>[2x]LSECKTGNGKNYRGTMSKTKNGITCQKWSSTSPHRPRFSPATHPSEGLEENYCRNPDNDPQGPWCYTTDPEKRYDYCDILECEEECMHCSGENYDGKISKTMSGLECQAWDSQSPHAHGYIPSKFPNKNLKKNYCRNPDRELRPWCFTTDPNKRWELCDIPRCTTPPPSSGPTYQCLKGTGENYRGNVAVTVSGHTCQHWSAQTPHTHERTPENFPCKNLDENYCRNPDGK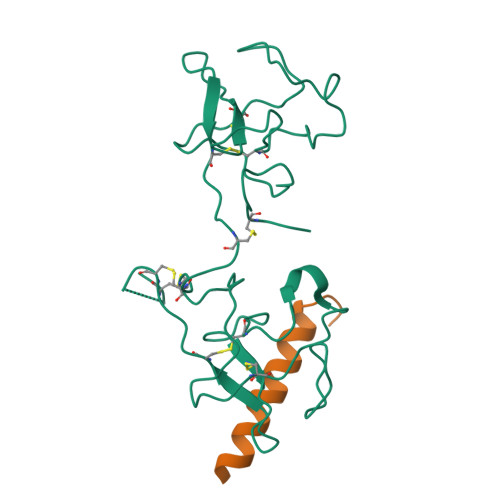RAP;>[2x]VEKLTADAELQRLKNERHEEAELERLKSEY> MTPNLQLYNKAYETLQGYGFPVISRKEMQQEIPYPFFVIKMPESNRSKYTFDSYSGDTNLVIDIWSVSDDLGHHDGLVKRCIDDLTPSVKTNDYDFEEDDTNITQLVDDTTNQELLHTSITIS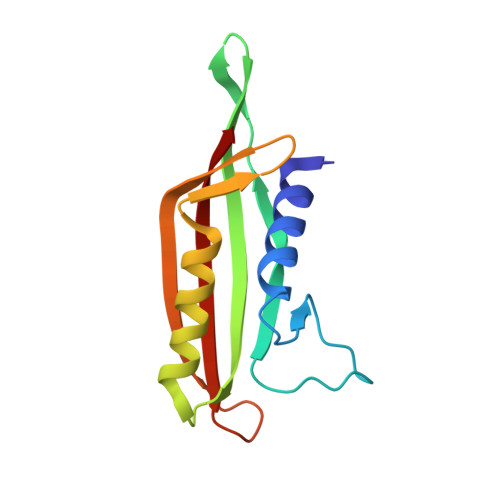YKTF>[2x]MSAIENFDAHTPMMQQYLRLKAQHPEILLFYRMGDFYELFYDDAKRASQLLDISLTKRGASAGEPIPMAGIPYHAVENYLAKLVNQGESVAICEQIGDPATSKGPVERKVVRIVTPGTISDEALLQERQDNLLAAIWQDSKGFGYATLDISSGRFRLSEPADRETMAAELQRTNPAELLYAEDFAEMSLIEGRRGLRRRPLWEFEIDTARQQLNLQFGTRDLV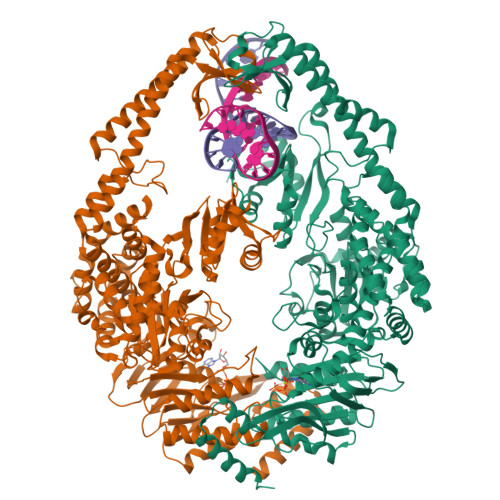GFGVENAPRGLCAAGCLLQYAKDTQRTTLPHIRSITMEREQDSIIMDAATRRNLEITQNLAGGAENTLASVLDCTVTPMGSRMLKRWLHMPVRDTRVLLERQQTIGALQDFTAGLQPVLRQVGDLERILARLALRTARPRDLARMRHAFQQLPELRAQLETVDSAPVQALREKMGEFAELRDLLERAIIDTPPVLVRDGGVIASGYNEELDEWRALADGATDYLERLEVRERERTGLDTLKVGFNAVHGYYIQISRGQSHLAPINYMRRQTLKNAERYIIPELKEYEDKVLTSKGKALALEKQLYEELFDLLLPHLEALQQSASALAELDVLVNLAERAYTLNYTCPTFIDKPGIRITEGRHPVVEQVLNEPFIANPLNLSPQRRMLIITGPNMGGKSTYMRQTALIALMAYIGSYVPAQKVEIGPIDRIFTRVGAADDLASGRSTFMVEMTETANILHNATEYSLVLMDEIGRGTSTYDGLSLAWACAENLANKIKALTLFATHYFELTQLPEKMEGVANVHLDALEHGDTIAFMHSVQDGAASKSYGLAVAALAGVPKEVIKRARQKLRELESIS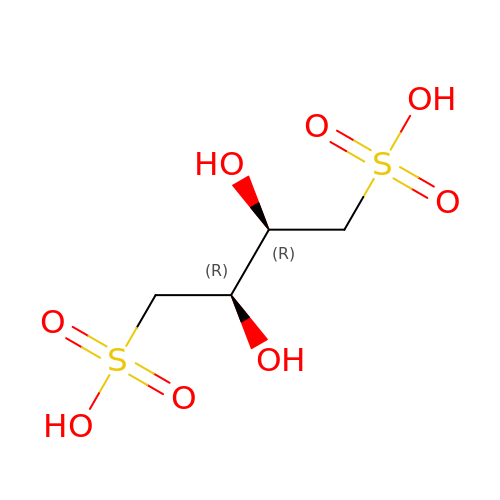(2R,3R)-2,3-bis(oxidanyl)butane-1,4-disulfonic acid | C4 H10 O8 S2 | HLYMICSVYBDBOV-IMJSIDKUSA-N Sampatrilat-Asp 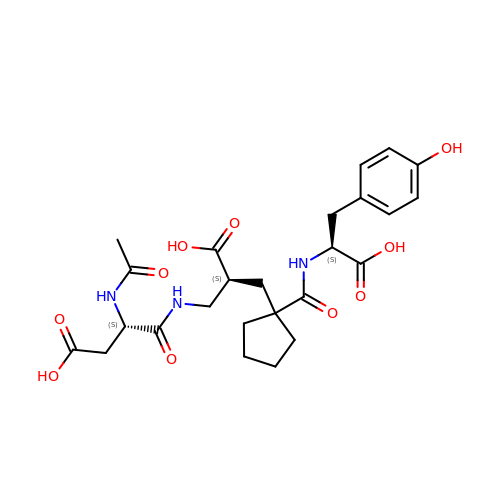| C25 H33 N3 O10 | ZQIWHIVXBQEYTN-WDSOQIARSA-N ATP synthases use a transmembrane electrochemical proton motive force (pmf) to generate adenosine triphosphate (ATP) from adenosine diphosphate (ADP) and inorganic phosphate (Pi). ATP synthases are macromolecular machines consisting of an ATP-hydrolysis-driven F1 motor and a proton-translocation-driven FO motor. The F1 and FO motors oppose each other’s action on a shared rotor subcomplex and are held stationary relative to each other by a peripheral stalk. In Saccharomyces cerevisiae, the FO region contains subunits a, e, f, g, i/j, k, 8, part of subunit b, and the c10-ring of the rotor, while the F1 region includes a trimer of catalytic subunit αβ pairs and subunits γ, δ, and ε from the rotor.

To test the hypothesis that the peripheral stalk of ATP synthase deforms under strain, we next added ATP to the preparation and froze cryoEM specimens. Classification of the resulting dataset yielded maps showing six different F1 states, corresponding to the catalytic and binding dwell structures from each of the three main rotational states. Subclassification of these populations separated each catalytic and each binding state into conformations with increasing rotation of the rotor relative to subunit a, and increasingly strained peripheral stalks, designated as ‘a’, ‘b’, ‘c’, etc. Overall, 27 unique conformations were identified: State 1binding(a to d), State 1catalytic(a to h), State 2binding(a to b), State 2catalytic(a to e), State 3binding(a to c), and State 3catalytic(a to e). Without ATP and during ATP hydrolysis, the left-handed curvature of the peripheral stalk remains the most highly populated conformation of the enzyme. Notably, the most strained conformation of some of the states show less rotation of the c-ring in the ATP hydrolysis direction than less strained conformations of the preceding state (shaded areas). The same apparent ‘backstepping’ can be seen at the transition from State 3catalytic → State 3binding, and State 2binding → State 1catalytic. This backstepping of the c-ring would bend the peripheral stalk in the opposite direction of the applied force and is physically unlikely. Therefore, the unstrained conformations appear to show inactive complexes that are not part of the rotary sequence during substrate turnover.

>[10x]MQLVLAAKYIGAGISTIGLLGAGIGIAIVFAALINGVSRNPSIKDTVFPMAILGFALSEATGLFCLMVSFLLLFGV;>ASTKAQPTEVSSILEERIKGVSDEANLNETGRVLAVGDGIARVFGLNNIQAEELVEFSSGVKGMALNLEPGQVGIVLFGSDRLVKEGELVKRTGNIVDVPVGPGLLGRVVDALGNPIDGKGPIDAAGRSRAQVKAPGILPRRSVHEPVQTGLKAVDALVPIGRGQRELIIGDRQTGKTAVALDTILNQKRWNNGSDESKKLYCVYVAVGQKRSTVAQLVQTLEQHDAMKYSIIVAATASEAAPLQYLAPFTAASIGEWFRDNGKHALIVYDDLSKQAVAYRQLSLLLRRPPGREAYPGDVFYLHSRLLERAAKLSEKEGSGSLTALPVIETQGGDVSAYIPTNVISITDGQIFLEAELFYKGIRPAINVGLSVSRVGSAAQVKALKQVAGSLKLFLAQYREVAAFAQFGSDLDASTKQTLVRGERLTQLLKQNQYSPLATEEQVPLIYAGVNGHLDGIELSRIGEFESSFLSYLKSNHNELLTEIREKGELSKELLASLKSATESFVATF[3x];>[3x]ASAAQSTPITGKVTAVIGAIVDVHFEQSELPAILNALEIKTPQGKLVLEVAQHLGENTVRTIAMDGTEGLVRGEKVLDTGGPISVPVGRETLGRIINVIGEPIDERGPIKSKLRKPIHADPPSFAEQSTSAEILETGIKVVDLLAPYARGGKIGLFGGAGVGKTVFIQELINNIAKAHGGFSVFTGVGERTREGNDLYREMKETGVINLEGESKVALVFGQMNEPPGARARVALTGLTIAEYFRDEEGQDVLLFIDNIFRFTQAGSEVSALLGRIPSAVGYQPTLATDMGLLQERITTTKKGSVTSVQAVYVPADDLTDPAPATTFAHLDATTVLSRGISELGIYPAVDPLDSKSRLLDAAVVGQEHYDVASKVQETLQTYKSLQDIIAILGMDELSEQDKLTVERARKIQRFLSQPFAVAEVFTGIPGKLVRLKDTVASFKAVLEGKYDNIPEHAFYMVGGIEDVVAKAEKLAAEAN;> ATLKEVEMRLKSIKNIEKITKTMKIVASTRLSKAEKAKISAKKMDEAEQLFYKNAETKNLDVEATETGAPKELIVAITSDKGLCGSIHSQLAKAVRRHLNDQPNADIVTIGDKIKMQLLRTHPNNIKLSINGIGKDAPTFQESALIADKLLSVMKAGTYPKISIFYNDPVSSLSFEPSEKPIFNAKTIEQSPSFGKFEIDTDANVPRDLFEYTLANQMLTAMAQGYAAEISARRNAMDNASKNAGDMINRYSILYNRTRQAVITNELVDIITGASSLG;> AEAAAASSGLKLQFALPHETLYSGSEVTQVNLPAKSGRIGVLANHVPTVEQLLPGVVEVMEGSNSKKFFISGGFATVQPDSQLCVTAIEAFPLESFSQENIKNLLAEAKKNVSSSDAREAAEAAIQVEVLENLQSVLK;> SAWRKAGISYAAYLNVAAQAIRSSLKTELQTASVLNRSQTDAFYTQYKNGTAASEPTPITK;> ASKAAAPPPVRLFGVEGTYATALYQAAAKNSSIDAAFQSLQKVESTVKKNPKLGHLLLNPALSLKDRNSVIDAIVETHKNLDGYVVNLLKVLSENNRLGCFEKIASDFGVLNDAHNGLLKGTVTSAEPLDPKSFKRIEKALSASKLVGQGKSLKLENVVKPEIKGGLIVELGDKTVDLSISTKIQKLNKVLEDSI;> SPLDQFEIRTLFGLQSSFIDLSCLNLTTFSLYTIIVLLVITSLYTLTNNNNKIIGSRWLISQEAIYDTIMNMTKGQIGGKNWGLYFPMIFTLFMFIFIANLISMIPYSFALSAHLVFIISLSIVIWLGNTILGLYKHGWVFFSLFVPAGTPLPLVPLLVIIETLSYFARAISLGLRLGSNILAGHLLMVILAGLTFNFMLINLFTLVFGFVPLAMILAIMMLEFAIGIIQGYVWAILTASYLKDAVYLH;> NDESILLLTFLGFTGLVAKYLAPAYKDFADARMKKVSDVLNASRNKHVEAVKDRIDSVSQLQNVAETTKVLFDVSKETVELESEAFELKQKVELAHEAKAVLDSWVRYEASLRQLEQRQLAKSVISRVQSELGNPKFQEKVLQQSISEIEQLLSK;> SLAKSAANKLDWAKVISSLRITGSTATQLSSFKKRNDEARRQLLELQSQPTEVDFSHYRSVLKNTSVIDKIESYVKQYKPVKIDASKQLQVIESFEKHAMTNAKETESLVSKELKDLQSTLDNIQSARPFDELTVDDLTKIKPEIDAKVEEMVKKGKWDVPGYKDRFGNLNVM;> VSTLIPPKVVSSKNIGSAPNAKRIANVVHFYKSLPQGPAPAIKANTRLARYKAKYFDGDNASGKPLWHFALGIIAFGYSMEYYFHLRHHKGAEEH;> NVIQDLYLRELKDTKLAPSTLQDAEGNVKPWNPPQKPNLPELELQGPEALKAYTEQNVETAHVAKESEEGESEPIEEDWLVLDDAEETKESH;> MLKRFPTPILKVYWPFFVAGAAVYYGMSKAADLSSNTKEFINDPRNPRFAKGGKFVEVD;> MPQLVPFYFMNQLTYGFLLMITLLILFSQFFLPMILRLYVSRLFISKL> EMPVDRILEAELAVEQKSDQGVEGPGGTGGSGSSPNDPVTNICQAADKQLFTLVEWAKRIPHFSSLPLDDQVILLRAGWNELLIASFSHRSIDVRDGILLATGLHVHRNSAHSAGVGAIFDRVLTELVSKMRDMRMDKTELGCLRAIILFNPDAKGLSNPSEVEVLREKVYASLETYCKQKYPEQQGRFAKLLLRLPALRSIGLKCLEHLFFFKLIGDTPIDTFLMEMLEAPHQLA;> MSPEQLGMIEKLVAAQQQCNRRSFSDRLRVTPWPMAPDPHSREARQQRFAHFTELAIVSVQEIVDFAKQLPGFLQLSREDQIALLKTSAIEVMLLETSRRYNPGSESITFLK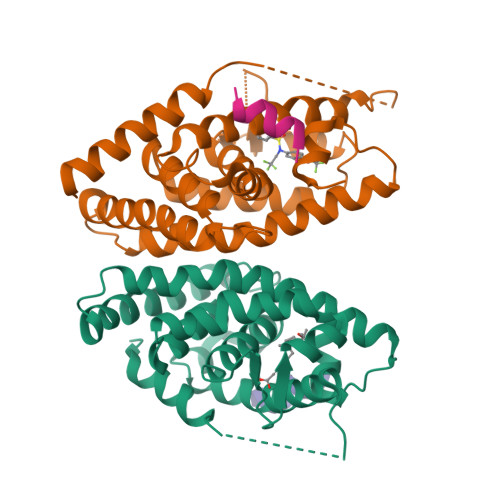DFSYNREDFAKAGLQVEFINPIFEFSRAMNELQLNDAEFALLIAISIFSADRPNVQDQLQVERLQHTYVEALHAYVSIHHPHDRLMFPRMLMKLVSLRTLSSVHSEQVFALRLQDKKLPPLLSEIWDVHE;>HKILHRLLQD[2x]> XQFEEI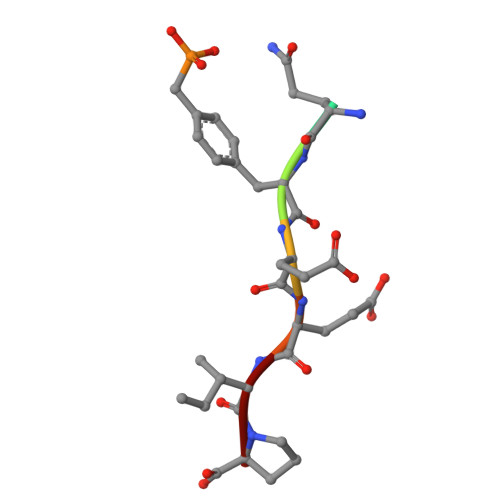P> AAQTNAPWGLARISSTSPGTSTYYYDESAGQGSCVYVIDTGIEASHPEFEGRAQMVKTYYYSSRDGNGHGTHCAGTVGSRTYGVVKKTQLFGVKVLDDNGSGQYSTIIAGMDFVASDKNNRNCPKGVVASLSLGGGYSSSVNSAAARLQSSGVMVAVAAGNNNADARNYSPASEPSVCTVGASDRYDRRSSFSNYGSVLDIFGPGTSILSTWIGGSTRSISGTSMATPHVAGLAAYLMTLGKTTAASACRYIADTANKGDLSNIPFGTVNLLAY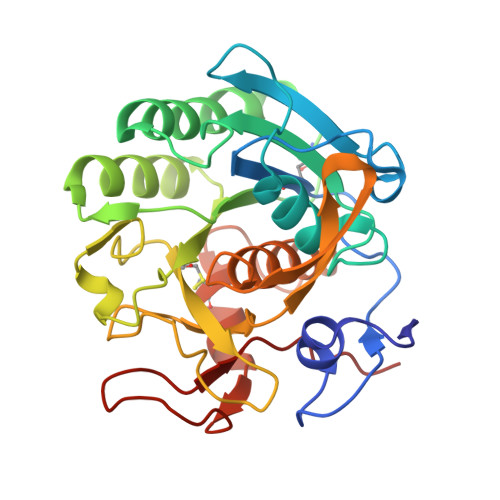NNYQA>[2x]DNYRCPNPGDAFECFESDATARFCVSGKRGAYVICSKCRRKYEFCA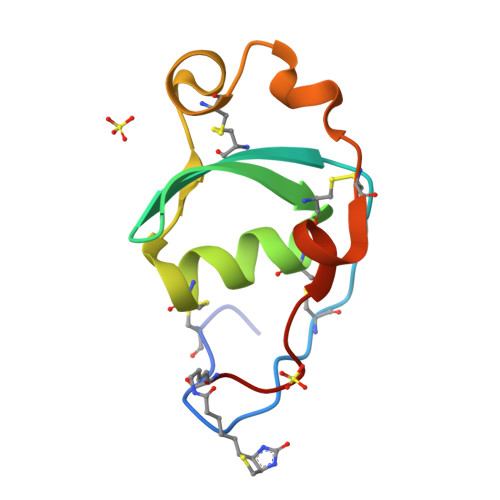NGAKVSKRPEVECRADWASTECTSENSDVPSVMKX> GPGSGDVCFHCNRVIEGDV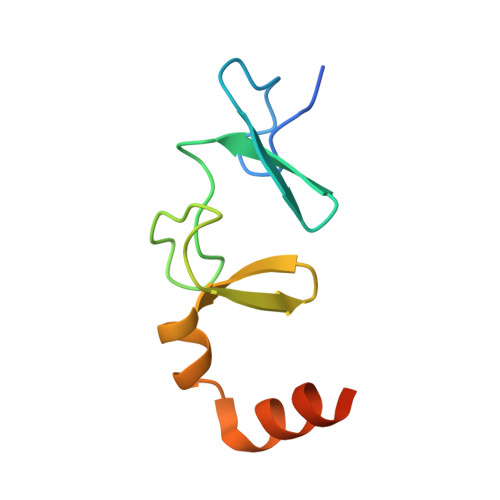VSALNKAWCVNCFACSTCNTKLTLKNKFVEFDMKPVCKKCYEKFPLELKKRLKKLAETLGRK> MKQYLELMQKVLDEGTQKNDRTGTGTLSIFGHQMRFNLQDGFPLVTTKRCHLRSIIHELLWFLQGDTNIAYLHENNVTIWDEWADENGDLGPVYGKQWRAWPTPDGRHIDQITTVLNQLKNDPDSRRIIVSAWNVGELDKMALAPCHAFFQFYVADGKLSCQLYQRAC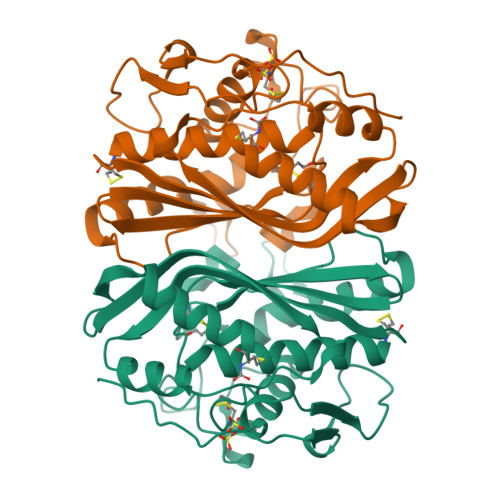DVFLGLPFNIASYALLVHMMAQQCDLEVGDFVWTGGDTHLYSNHMDQTHLQLSREPRPLPKLIIKRKPESIFDYRFEDFEIEGYDPHPGIKAPVAI> ELQARSRIKWAIDYITKYFFTEGIYLQKRQREQRLL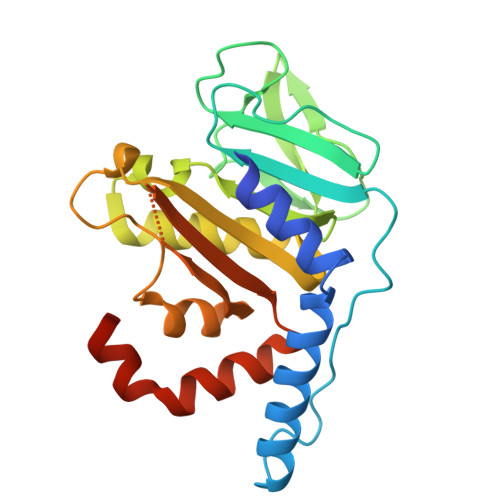ESYRAEGKLGEVQCRLMEEPPDRLHVLDVGSCFNPFSSAPHLEVTALDLCPATEDVLQADFLKVEVVPGIREPELEEGSVRRLPASHYECVIFSLLLEYMPSAEQRLQCCLQAYDLLLPEGILVLITPDSQHVGKNAHLMKNWRYSLARIGLLRVRFEKLPHISCMVFRKAISRELSQHWASIHREEGMCEEIRIPQDDS> SIYNSFYVYCKGP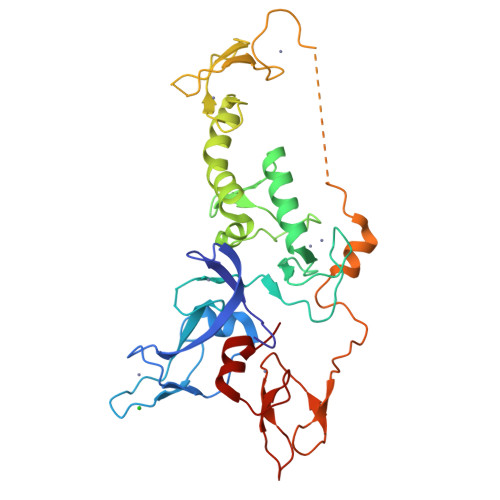CQRVQPGKLRVQCSTCRQATLTLTQGPSCWDDVLIPNRMSGECQSPHCPGTSAEFFFKCGAHPTSDKETPVALHLIATNSRNITCITCTDVRSPVLVFQCNSRHVICLDCFHLYCVTRLNDRQFVHDPQLGYSLPCVAGCPNSLIKELHHFRILGEEQYNRYQQYGAEECVLQMGGVLCPRPGCGAGLLPEPDQRKVTCEGGNGLGCGFAFCRECKEAYHEGECSAVFEASGTTTQAYRVDERAAEQARWEAASKETIKKTTKPCPRCHVPVEKNGGCMHMKCPQPQCRLEWCWNCGCEWNRVCMGDHWFDV>[2x]AMRQCAIYGKGGIGKSTTTQNLVAALAEMGKKVMIVGCDPKADSTRLILHSKAQNTIMEMAAEAGTVEDLELEDVLKAGYGGVKCVESGGPEPGVGCAGRGVITAINFLEEEGAYEDDLDFVFYDVLGDVVCGGWAMPIRENKAQEIYIVCSGEMMAMYAANNISKGIVKYANSGSVRLGGLICNSRNTDREDELIIALANKLGTQMIHFVPRDNVVQRAEIRRMT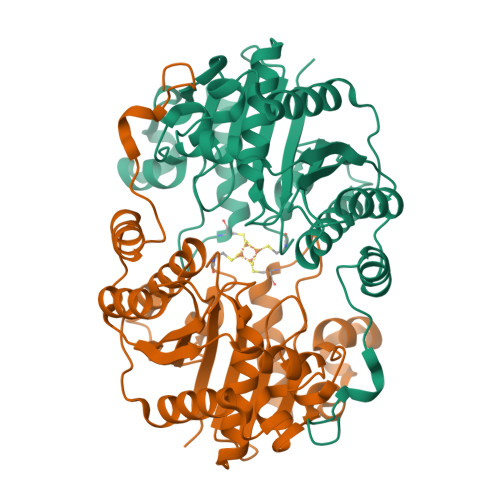VIEYDPKAKQADEYRALARKVVDNKLLVIPNPITMDELEELLMEFGIMEVEDESIVGKTAEEV(2Z,5Z)-2-[(4-ethylphenyl)imino]-3-methyl-5-[(2-{[4-(1H-tetrazol-5-yl)phenyl]amino}pyridin-4-yl)methylidene]-1,3-thiazolidin-4-one 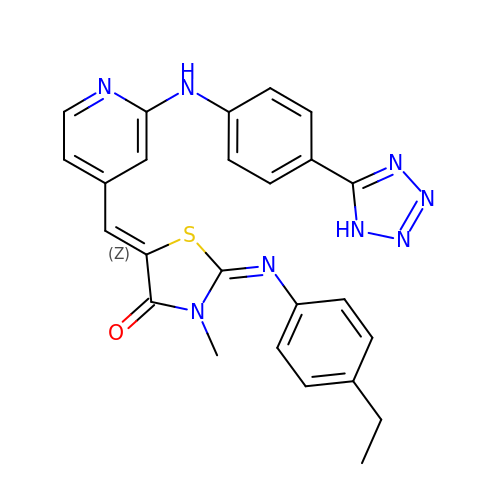| C25 H22 N8 O S | WWPZBBQLQAEXGE-ZMSDRGEISA-N> MXQ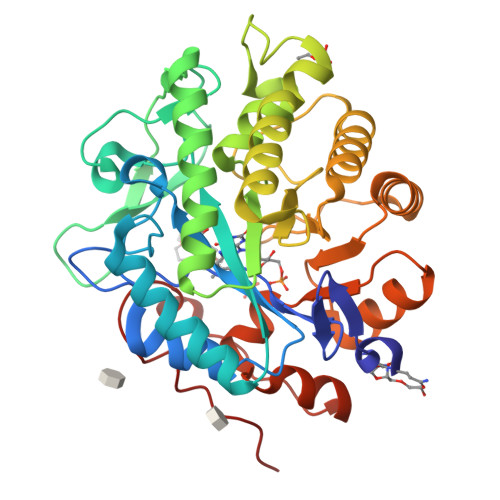SLFQPITLGALTLKNRIVMPPLTRSRASQPGDVANHMMAIYYAQRASAGLIVSEGTQISPTAKGYAWTPGIYTPEQIAGWRIVTEAVHAKGCAIFAQLWHVGRVTHPDNIDGQQPISSSTLKAENVKVFVDNGSDEPGFVDVAVPRAMTKADIAQVIADYRQAALNAMEAGFDGIELHAANGYLINQFIDSEANNRSDEYGGSLENRLRFLDEVVAALVDAIGAERVGVRLAPLTTLNGTVDADPILTYTAAAALLNKHRIVYLHIAEVDWDDAPDTPVSFKRALREAYQGVLIYAGRYNAEKAEQAINDGLADMIGFGRPFIANPDLPERLRHGYPLAEHVPATLFGGGEKGLTDYPTYQA> HHTFEYGDG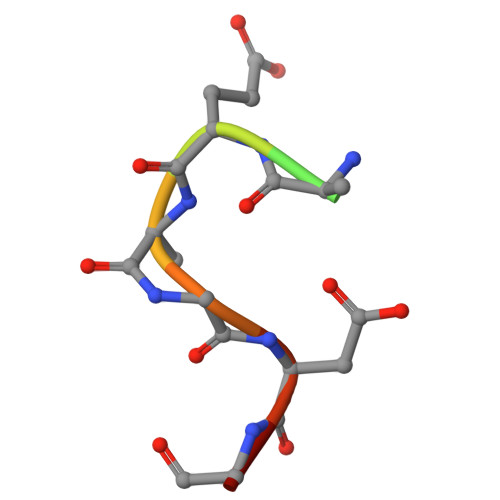I> GAMESLPVIAAPSMWTRPQIKDFKEKIQQDADSVITVGRGEVVTVRVPTHEEGSYLFWEFATDNYDIGFGVYFEWTDSPNTAVSVHVSESSDDDEEEEENIGCEEKAKKNANKPLLDEIVPVYRRDCHEEVYAGSHQYPGRGVYLLKFDNSYSLWRSKSVYYRVYYTR;> GSGSGTPAPDAINDALRSADSQEA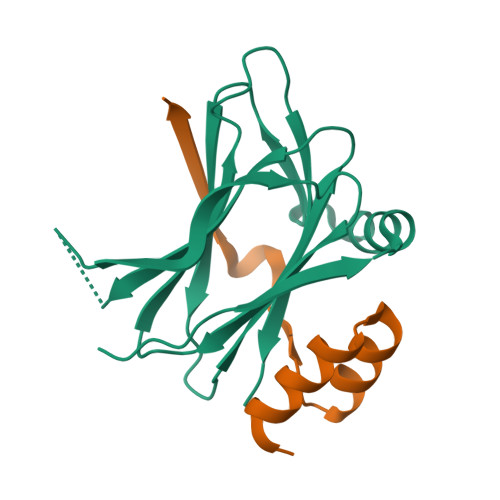RDACQKKGWIVIHPSNELVVEKHISR In summary, our study demonstrates that PH0208 protein would function as a purine nucleotide dependent R15Pi enzyme and not as a homologue of the regulatory subunit of eIF2B. In NMP degradation pathway, R15Pi catalyzes the conversion of ribose-1,5-bisphosphate (R15P, substrate) into ribulose-1,5-bisphosphate (RuBP, product) in an adenosine 5′-monophosphate (AMP)-dependent manner. AMP acts as an activator of R15Pi and in its absence the enzymatic activity has been found to decline dramatically. Monomer of PH0208 protein consists of an N-terminal α-helical domain (residues 1–122) and a C-terminal α-β-α sandwich domain (residues 123–324).

In order to verify the role of the catalytic residues in PH0208 protein, the residue Cys135 was mutated to serine. The mutation led to the formation of a catalytically inactive protein which lost the ability to convert the substrate into product and thus, held the substrate in the active site pocket. The substrate molecule (R15P) binds to the active site of PH0208-C135S in a manner similar to that of the wild type (WT) protein. Therefore, binding affinity was studied using the mutant proteins, PH0208-C135S and PH0208-D204N in which case the heat change would be solely due to ligand binding. The analysis shows that both PH0208-C135S and PH0208-D204N proteins bind to R15P with high affinity with equilibrium dissociation constants (Kd) of 13.8 and 10 μM, respectively. On the contrary, the PH0208-C135S and PH0208-D204N bind the product (RuBP) with negative ∆H value for the binding peaks indicating an exothermic reaction. The mutants formed strong interactions with RuBP with Kd values of 7.5 and 7.2 μM, respectively, which corresponds to the binding affinity of the substrate. The residues Cys135 and Asp204, known to be absolutely conserved in R15Pi enzyme and essential for the catalysis of R15P (substrate) to RuBP (product) are also conserved in PH0208 protein. Mutation of these two residues in PH0208 protein led to the inhibition of the isomerization of the substrate into product.

>[3x]MGAMIVKEVYETAEKIKSMEIRGAGRIARAAAQALMIQAEKSKAKEPEELWNELKVASKILYNTRPTAVSLPNALRYVMHRVKAAYLGGADLETLRFTAINSAKEFIYNSEKAIERIGEIGAKRIEDGDIIMTHSHSKAAISVMKKAFEQGKNIKVIVTETRPKWQGKITAKELASYGIPVIYIVDSAARHYMKMTDKVVMGADSITANGAVINKIGTSLIALTAKEHRVWVMIAAETYKFHPATMLGQLVEIEMRDPTEVIPEEELRTWPKNIEVWNPAFDVTPPEYIDVIITERGIIPPYAAIDILKEEFGWALKYKEPWED>MAYPGHPGAGGGYYPGGYGGAPGGPAFPGQTQDPLYGYFAAVAGQDGQIDADELQRCLTQSGIAGGYKPFNLETCRLMVSMLDRDMSGTMGFNEFKELWAVLNGWRQHFISFDTDRSGTVDPQELQKALTTMGFRLSPQAVNSIAKRYSTN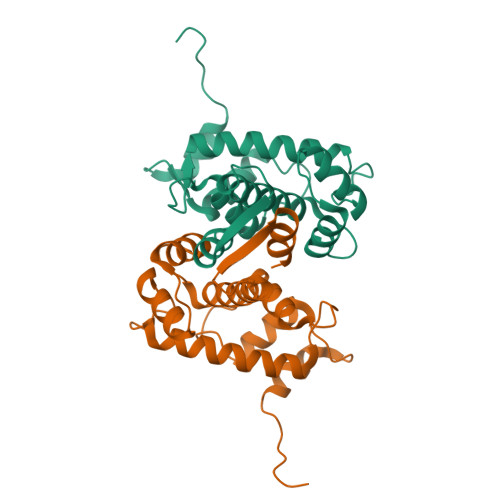GKITFDDYIACCVKLRALTDSFRRRDTAQQGVVNFPYDDFIQCVMSV[2x]> MAFSAGAESLLHQAREIQDEELRRFCSRVTKLLQEAPGPATVDALQRLFLIVSATKYPRRLEKMCVDLLQTTLCLPASPEQLQVLCAAILREMSPFNDLALSCDHTPNTRQLSLVASVLLAQGDRKGEIRCVSQRIFKILENRQPEGPSVRPLLPILSKVIGLAPGILMEDQTNLLSKRLVDWLRYASIQQGLPYSGGFFSTPRTRQPGPITEVDGAVASDFFTVLSTGQHFTEDQWVNMQAFSMLRKWLLHSGPEDPCSPDADDKSELEGSTLSVLSAASTASRLLPPRE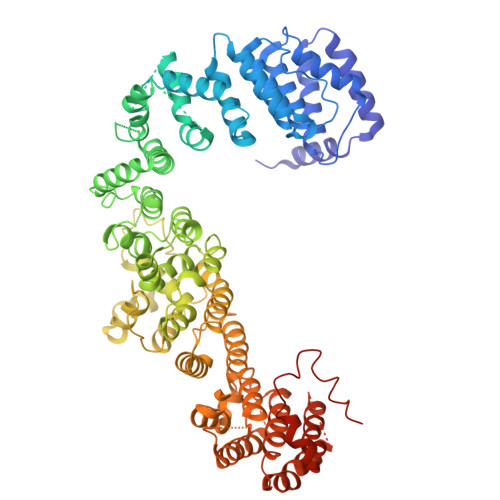RLREVAFEYCQRLLEQSNRRALRKGDSDLQKACLVEAVSVLDVLCRQDPSFLYRTLSCLKALHRRLGEDPGSERALVPLAQFFLNHGEAAAMDAEAVYGQLLRGLPSERFHSPTLAFEVIHFCTHNLALFDSHFLSLLRLSFPSLFKFLAWNSPPLTAEFVVLLPALVDAGTAVEMLHALLDLPCLTAALDLQLRSTQTPSERLLWDISLRVPSCLEAFQDPQFQGLFRHLLRTKASGSTERLTPLHQVLKPMASCARVTQCAEAVPVLLQAFFSAVTQTADGALINQLALLLLERSDSLYPVPQYEARVHGVLSSQLLVLCKLKPSLVVELSRELLEFVGSVSSIHSRASVFTCVVWAIGEYLSVTWDKRCTAEQINKFFEALEALLFEVTQSRPLADLPCCPPEVVTALMTTLTKLASRSQDLIPRVSLFLSKMRTLAQNPATSSVHSEEGAESIRTRASELLTLLKMPSVAQFVFTPPAGVCQPRYHRDTNVALPLALRTVSRLVEKEAGLLPG2-chloro-N-[4-(4-methoxyphenyl)-1,3-thiazol-2-yl]-N-(3-methoxypropyl)acetamide 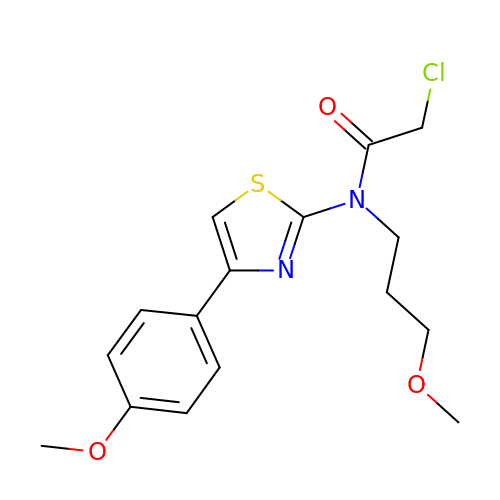| C16 H19 Cl N2 O3 S | KZMAWJRXKGLWGS-UHFFFAOYSA-N[FeFe]-hydrogenases represent one of natures’ most effective classes of redox enzymes catalyzing the reversible reduction of protons to dihydrogen (H2) at turnover frequencies of up to 9000 s-11–3. With their low catalytic over-potential, [FeFe]-hydrogenases represent excellent models for a regenerative and likewise economically feasible H2 production. Their active center (“H-cluster”) can be structured into a standard [4Fe-4S]-cluster ([4Fe]H) and a diiron site ([2Fe]H). Theoretical studies suggest that the most probable PT pathway comprises of strictly conserved residues E282, S319, E279, and C299 (from surface to H-cluster, numbering corresponds to CpI), including two protein-bound water molecules (Wat826, Wat1120 4XDC19, chain B) located between E279 and C29915,16,20. In this study, site-directed mutagenesis (SDM) is used to investigate the PT pathway of two [FeFe]-hydrogenases, namely CpI and HydA1, which represent the largest (M3) and smallest (M1) type of monomeric [FeFe]-hydrogenases, respectively.

Crystallization of HydA1 exclusively succeeded for apo-protein, which carries the [4Fe]H-cluster but lacks the [2Fe]H-site. Variants of HydA1 apo-protein were crystallized in space group P32 2 1, with a single chain in the asymmetric unit. However, comparisons of crystal structures of CpI apo- and holo-protein with apo-HydA1 demonstrated that a lack of cofactor does not affect the configuration of the putative PT pathway. In the corresponding HydA1-variant E141Q, the glutamine residue precisely adopts the conformation of the glutamic acid residue in HydA1 wild type. While glutamine occupies the entire space of the native carboxyl group and thus clearly interrupts the putative PT pathway, an exchange to alanine may support additional H2O molecules to bridge the gap.

> MAAPAAEAPLSHVQQALAELAKPKDDPTRKHVCVQVAPAVRVAIAETLGLAPGATTPKQLAEGLRRLGFDEVFDTLFGADLTIMEQGSELLHRLTEHLEAHPHSDEPLPMFTSCCPGWIAMLEKSYPDLIPYVSSCKSPQMMLAAMVKSYLAEKKGIAPKDMVMVSIMPCTRKQSEADRDWFCVDADPTLRQLDHVITTVELGNIFKERGINLAELPEGEWDNPMGVGSGAGVLFGTTGGVMEAALRTAYELFTGTPLPRLSLSEVRGMDGIKETNITMVPAPGSKFEELLKHRAAARAEAAAHGTPGPLAWDGGAGFTSEDGRGGITLRVAVANGLGNAKKLITKMQAGEAKYDFVEIMACPAGCVGGGGQPRSTDKAITQKRQAALYNLDEKSTLRRSHENPSIRELYDTYLGEPLGHKAHELLHTHYVAGGVEEKDEKKSAWSHPQFEK>[4x]MHHHHHHENLYFQGASVLVASNRGPVSYVRGEDGELDARRGGGGLVSGLSAVSSQDSLWVCAALGEGDREAVRRGIGEPGVRMLDIAPDVYADAYNGIANSVLWFLHHHLYDIPREPVFDAAFRHRWEAYRAYNRAFAEALAAAADEGAAVLVQDYHLALVPGQLRELRPDLRIGHFTHTPWASPEYFRMLPADIGDELLRGMLGADELGFHTSAWASAFLSCAGGEQPRTRVRVHPLGVDAEELRALAHRPQVDERLARLREEVGDRKTIVRVDRTELSKNILRGLLAYRELLTVHPEWRDRVVHLASAYPSRQDLAAYRAYTASVTELAAEINAEFGTADWQPVLVSVEDDFTRSLAAYRLADVALVNPVRDGMNLVAKEIPVVSDAGCALVLSTGAGAYEELKEDALTVHPYDVSETAEALHTALTMPPPERADRTKRLASAATALPPQRWFLNQLEGLSDA

The only route for the de novo biosynthesis of trehalose in S. venezuelae is via trehalose 6-phosphate. OtsA (α,α-trehalose-phosphate synthase) is responsible for the formation of this metabolic intermediate from an NDP-glucose donor and glucose 6-phosphate as the acceptor. In all cases, trehalose 6-phosphate is dephosphorylated by OtsB (EC 3.1.3.12, trehalose-6-phosphate phosphohydrolase) to give trehalose. We have now shown that S. venezuelae OtsA has a preference for GDP-glucose as the donor, as has been reported for OtsA enzymes from other Streptomyces species and other actinomycetes, such as Rubrobacter xylanophilus.

To establish the structural basis for the donor specificity of S. venezuelae OtsA, the recombinant enzyme was crystallized. Crystals diffracted to 1.95 Å, allowing the protein structure to be solved using molecular replacement. Four copies of the S. venezuelae OtsA protein were present in the asymmetric unit. Consistent with the size observed in solution, the biological unit appeared to be a dimer. The fold comprised twin Rossman-like β/α/β domains in a GT-B configuration. A molecule of MES buffer is bound in a cleft between the two domains of S. venezuelae OtsA in what is likely to be the active site, by analogy with the E. coli enzyme. Attempts to obtain a structure of the S. venezuelae enzyme with either GDP or GDP-glucose bound were unsuccessful. By contrast, the equivalent residues that define the donor base specificity of VldE, which uses GDP-valienol, are similar in S. venezuelae OtsA. Our structure of S. venezuelae OtsA most closely resembles the open conformations despite not having any ligands bound. In addition, there is a lack of electron density associated with a loop comprising amino acids 18–22 (peptide sequence GEDGE) of the S. venezuelae enzyme, implying disorder in this region.> GAQVSRQNVGTHSTQNMVSNGSSINYFNINYFKDAASSGASRLD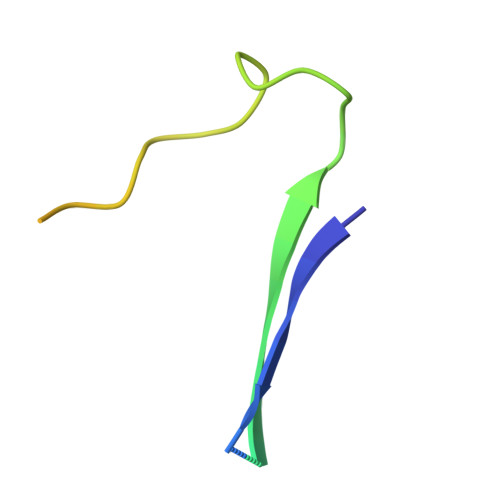FSQDPSKFTDPVKDVLEKGIPTLQ>[4x]MFKGVYPAIITPFKNKE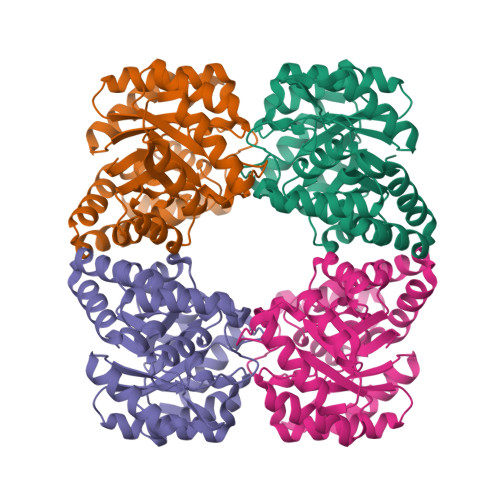VDFDGLEENINFLIENGVSGIVAVGTTGESPTLSHEEHKKVIEKVVDVVNGRVQVIAGAGSNCTEEAIELSVFAEDVGADAVLSITPYYNKPTQEGLRKHFGKVAESINLPIVLYNVPSRTAVNLEPKTVKLLAEEYSNISAVKEANPNLSQVSELIHDAKITVLSGNDELTLPIIALGGKGVISVVANIVPKEFVEMVNYALEGDFEKAREIHYKLFPLMKAMFIETNPIPVKTALNMMGRPAGELRLPLCEMSEEHKKILENVLKDLGLI> ACTKNAIAQTGFNKDKYFNGDVWYVTDYLDLEPDDVPKRYCAALAAGTASGKLKEAL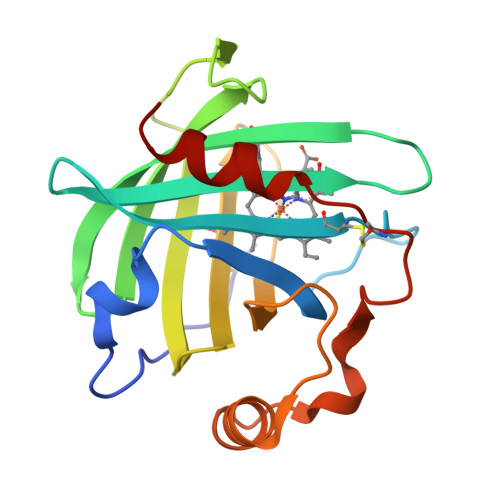YHYDPKTQDTFYDVSELQVESLGKYTANFKKVDKNGNVKVAVTAGNYYTFTVMYADDSSALIHTCLHKGNKDLGDLYAVLNRNKDAAAGDKVKSAVSAATLEFSKFISTKENNCAYDNDSLKSLLTK>MGSSHHHHHHSGGLVPRGSMSNQLERGPVRTPHADVLLASVGERGVLCDFYDEGAADTYRDLIQDADGTSEAREFATRTGPVSGPVLELAAGMGRLTFPFLDLGWEVTALELSTSVLAAFRKRLAEAPADVRDRCTLVQGDMSAFALDKRFGTVVISSGSINELDEADRRGLYASVREHLEPGGKFLLSLAMSEAAESEPLERKQELPGRSGRRYVLHVRHLPAEEIQEITIHPADETTDPFVVCTHRRRLLAPDQVVRELVRSGFDVIAQTPFASGGAGRKDMVLVEAVM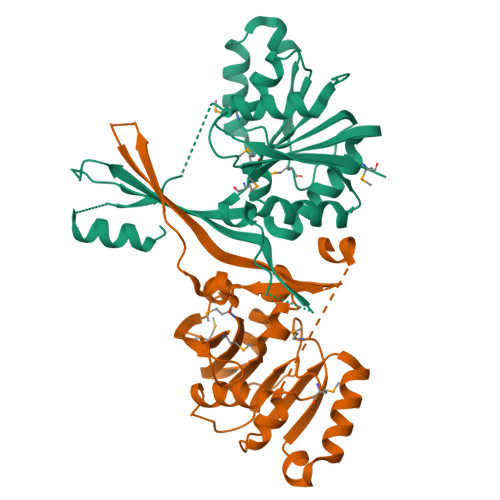PGATADAR[2x]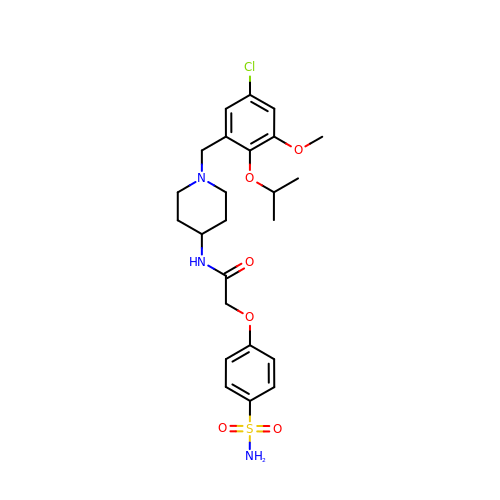N-{1-[5-chloro-3-methoxy-2-(1-methylethoxy)benzyl]piperidin-4-yl}-2-(4-sulfamoylphenoxy)acetamide | C24 H32 Cl N3 O6 S | QVZLZLJHCAPQQC-UHFFFAOYSA-N4-(2-aminoethyl)-2-ethylphenol | C10 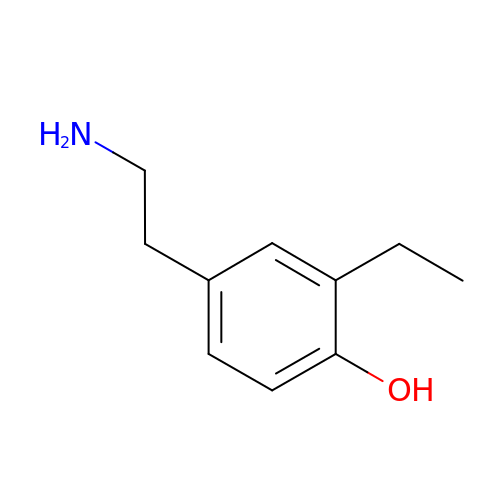H15 N O | LDAFQVRTSOETPE-UHFFFAOYSA-N> ACCAACTTCCCGTCCGACGGTCCGGTTATGCAGAAAAAAACCATGGGTTGGGAAGCTTCCACCGAACGTATGTACCCGGAAGACGGTGCTCTGAAAGGTGAAATCAAAATGCGTCTGAAACTGAAAGACGGTGGTCACTACGACGCTGAAGTTAAAACCACCTACATGGCTAAAAAACCGGTTCAGCTGCCGGGTGCTTACAAAACCGACATCAAACTGGACATCACCTCCCACAACGAAGACTACACCATCGTTGAACAGTACGAACGTGCTGAAGGTCGTCACTCCACCGGTGCTTAATAACGCTGATAGTGCTAGTGTAGATCGCTACTAGAGCCAGGCATCAAATAAAACGAAAGGCTCAGTCGAAAGACTGGGCCTTTCGTTTTATCTGTTGTTTGTCGGTGAACGCTCTCTACTAGAGTCACACTGGCTCACCTTCGGGTGGGCCTTTCTGCGTTTATACGTCTCTCATTGACCGGGAGCGCCCTGTAGCGGCGCATTAAGCGCGGCGGGTGTGGTGGTTACGCGCAGCGTGACCGCTACACTTGCCAGCGCCCTAGCGCCCGCTCCCGGGATCGGAATTCCGGCCATCGCCCTGATAGACGGTTTTTCGCCCTTTGACGTTGGAGTCCACGTTCTTTAATAGTGGACTCTTGTTCCAAACTGGAACAACACTCAACCCTATCTCGGGCAAGCTTGTCACAGAGACGCAATACGCAAACCGCCTCTCCCCGCGCGTTGGCCGATTCATTAATGCAGCTGGCACGACAGGTTTCCCGACTGGAAAGCGGGCAGTGAGCGCAACGCAATTAATGTGAGTTAGCTCACTCATTAGGCACCCCAGGCTTTACACTTTATGCTTCCGGCTCGTATGTTGTGTGGAATTGTGAGCGGATAACAATTTCACACATACTAGAGAAAGAGGAGAAATACTAGATGGCTTCCTCCGAAGACGTTATCAAAGAGTTCATGCGTTTCAAAGTTCGTATGGAAGGTTCCGTTAACGGTCACGAGTTCGAAATCGAAGGTGAAGGTGAAGGTCGTCCGTACGAAGGTACCCAGACCGCTAAACTGAAAGTTACCAAAGGTGGTCCGCTGCCGTTCGCTTGGGACATCCTGTCCCCGCAGTTCCAGTACGGTTCCAAAGCTTACGTTAAACACCCGGCTGACATCCCGGACTACCTGAAACTGTCCTTCCCGGAAGGTTTCAAATGGGAACGTGTTATGAACTTCGAAGACGGTGGTGTTGTTACCGTTACCCAGGACTCCTCCCTGCAAGACGGTGAGTTCATCTACAAAGTTAAACTGCGTGGT;> CGTCAAAGGAACGCGCGGGGAGCTTGCCCGAGATACTCTAGTAGCTTTG;> ACTCCAAGTGTTGTTCCAGTTGTCTGGGACTGCGGGTGTAGT;> CCACTATTAAAGAACGTGGTCAGGGCTATCCGG;> TGCGTCTCTTATCCGGTGCCTAACAGA;> CGAACTCACATTAACTGCATTAATGAATCGGCCGC;> TGTTTAATTCCGGGGAGACGTATAAACGCAGAAGGTCCCATTTGAAACC;> GATGTCATACTGGATACCTTCGTACGTGGGTTGA;> CAAGTGGATGGCCGGAATTCCGATCCCGGGATTT;> TTTGCGGGCGCTAGGGTAACCACCACATTT;> TTTCCAGTCGGGAAACCTGTCGTGCCAGTTGCGTACACGTAGTCCT;> GGGTAACACCGTCTTAAAACGTTATTTGATGCCTGGTACATACGTT;> TTTCCCGCCGCGCTTAATGCGCAGTTTGATGTCGGTTTTGTTTT;> TTTACCGTCTTCGAAGTTCATATGCGCTC;> AAGGACAGTTTCAGGTAGGCAGGGCGCTCCCGGTCAATGA;> GGTCACGCTGCGCGCGCTGGGATGTCCTTTCAGTTCGAACTCG;> TTTAAGCACCCGGCAGCTGAACCGGTTTATGTCCCGCTAC;> TTTGTAGATGAACTCGGTAACAACACCTTT;> TGCAGGAGTTGGTACCACGC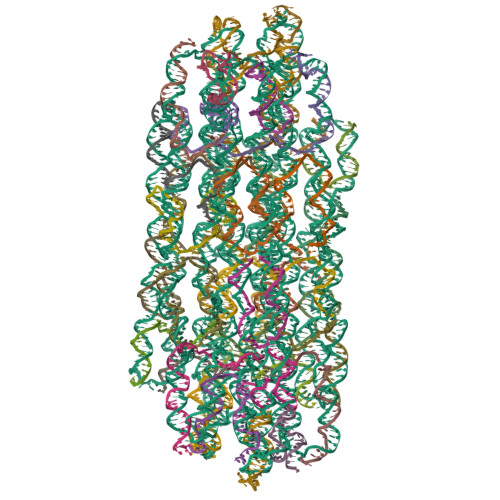AGTTTAACTTTTTT;> CCAGTGTGTTGTGGGAGGTGTTTAGCCATGTAGGTGGTTA;> GAGGAAGCCATCAAATTGTGTGACAAGAGGCGGTTTGCGTAT;> CTTCCATGTTATTATCAGACGTCGTAGTGACCACCGT;> TGACCGTTAACGGAACTTCGATTTTAGCGTGGAACAAGAGT;> GTTCACCGTAGCGACTCTTTGATAACGTCTTCG;> AGAGAGCAGGTGAGTAACCGGACCGTCGCATGGTT;> TCTAGTGAACCGGCCGGGGAAAAACCGTCTA;> CTTCGACTATCAGCACGAACTTTGAAACTTGACGACCTTCACCTTCACC;> TTTACGTTCGTACTGTTCAGGTGGAGTGACGACCTTTT;> TTTGACTGAGCCTTTCGTTAAAGGCCGTGTAAAACTGCCCGCTTTTTT;> TTTGACCACCTTTGGTAACCAAGCGAACGGCAGCGTTT;> TTTCGGAAGCATAAACAGTCTTTCTTT;> GCCTGGGCTCACAATTCCACACAACATACGAGCTTT;> GAGCTTAATGTGTGTAGTATTTCTCCTCGCATGAATCTACAC;> AGCACCGTCTTCCGGGCTCTAGACAAACAATGAGT;> CTTTCAGTTTTTCTGCTTAACTTCAGCGCATTTTGATTTCACTAGCAC;> CTTTCAGTTAGCACCACGATGGGACAG;> CGGTGGAAGCTTCCCAACCGACGGGAGAAGGCCCACCCGA> MLIIGERINGMFGDIKRAIQERDPAPVQEWARRQEEGGARALDLNVGPAVQDKVSAMEWLVEVTQEV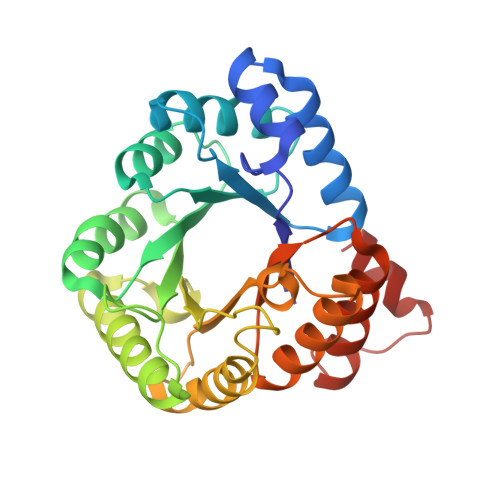SNLTLCLDSTNIKAIEAGLKKCKNRAMINSTNAEREKVEKLFPLAVEHGAALIGLTMNKTGIPKDSDTRLAFAMELVAAADEFGLPMEDLYIDPLILPANVAQDHAPEVLKTLQQIKMLADPAPKTVLGLSNVSQNCQNRPLINRTFLAMAMACGLDAAIADACDEALIETAATAEILLNQTVYCDSFVKMFKTR>[2x]MDIETIVNEFETRAGTLLRYYTGLLERSKVQPCCFKLYNDPFDMVYVMMNSKLFSHVYIKDCKVRQSFELASPKHTEGLIRSIEGHYVGYELHDGKQLS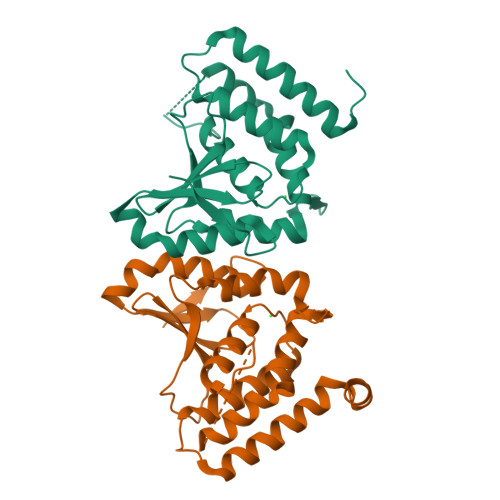ISDMMASQLFEDEYFMYGLQTYAESNNSDVFKCLENGFDTDTLEGIQSSNTDVIANIEMLYQLATGINEPVPELVEGLKLVTEFVQDENATQEDYKALERKLNDLKASYYSLSKLAAALEHHHHHH> MFGRSALCLAKRFRYNTKYPSLVSYNKLPWEILNHETPEFHMHVAPHYEQIMTLAASTHVPHIVGKKHLEMPPEHRLRLLPGMFYMLDGDSIPEGFTANRVLDPTALQYYGRLESLVAPVQAVRMLISDDLRIVCNSVTLQGPLQLPVASYASLASLEVVTNKASASFTLFHFVRPNRPPSELQLEKYYIHAPRAMALAEFNSTSNTSWEPKLQAPKRSKRVTPLPAYRPPQSYLMGLAERLAVVPGSSFGRRSLM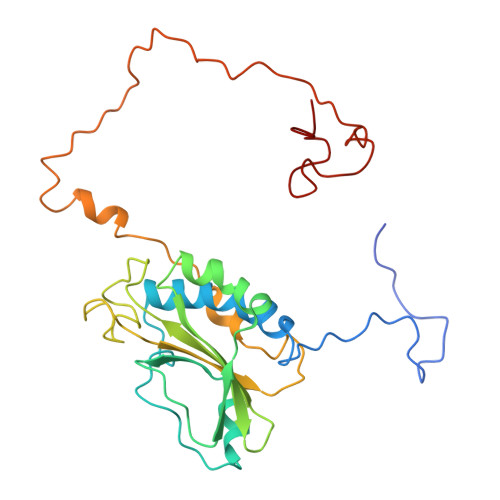WGHWF> EAIQTRAVINQHGTSETLVENFLGRAALVMMKDFEYKNHVTGTQKVQQNFFKWTINTRSYVQLRRKFELFTYIRFDSEITIVPTIRLYTSTGASYSGLPNLTLQAMFVPVGAPTPKSQDSYEWQSACNPSVFFKIDDPPARMTIPFMCINSAYGMFYDGFAGFEKTANGLYGINPANTMGNLCIRVVNAYQPVQYTITIRIYLKPKHIKAWVPRPPRTMPYMSIANTNYTGH;> VLQLKL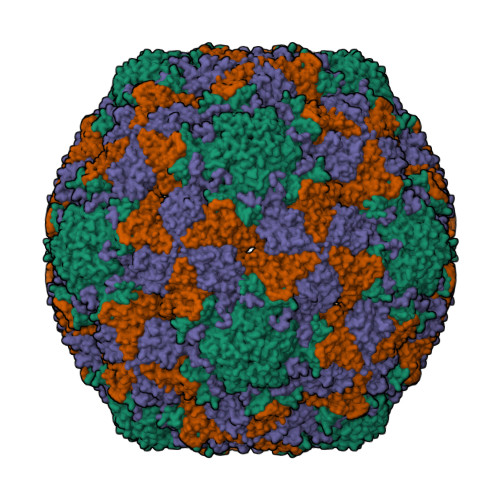GNSAIVTQEAANMCCAYGEWPSYLPDNEATAIDKPTQPETSTDRFYTLKSVKWEGTSTGWWWKLPDALNQTGMFGQNVQYHYLYRSGFLCHVQCNATKFHQGALLVVAIPEHQLGKYNTGTSASFDDVMKGKTGGVFTHPYVLDDGTSLACSLIFPHQWINLRTNNSATIMLPWMNCAPMDFALRHNQWTLAIIPVVPLNTSGGTTMVPITVSIAPMCCEFNGLRNAIT;> GVPTYLLPGSSQFMTTDDHSSAPAFPDFSPTPEIHIPGRVHNMLELVQVESMMEINNVAGSSGMERLRVEISVQTDMDALLFNIPLDIQLDGPLRSTLLANIARYYTHWSGSMEMTFMFCGSFMATGKVILCYTPPGGSCPTDRESAMLGTHIVWDFGLQSSITLVIPWISGSHFRMFNSDAKSINANVGYVTCFMQTNLIVPKEAATSTYIIGFAAAKNDFSLRLMRDSPDIGQSQQLE>GIDPFTESVLQSQATELLQKKAQLVSFKIQGIMKRIFMGANTLEKFLSDENSAINDTLKRRMLSEFLLANPHVLLVSAIYTNNNERVITAMSMDSKIAYPNTT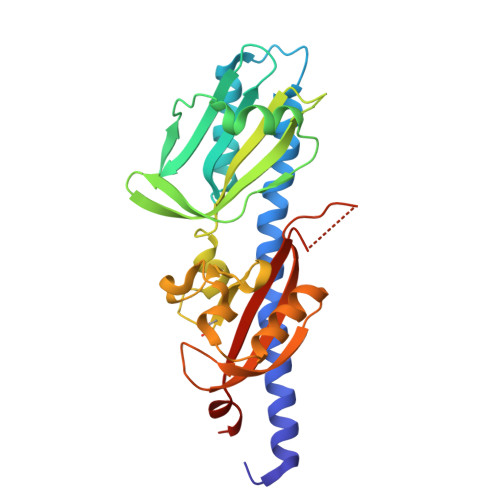LNENMTNQIRSLKSITHSDPYYKEVNGDKIYGMDITLPLMGKNQNAIGALNFFLNIDAFYTDVVGKKKSNTFLMGKDGRLLINPNREIQDKILSAINPDRRVAKAVEYYNQNEAGTLSYHSLSGNTETFLAIQPFDFFEEKGNNGNHWRWAIGKYVNKSLVFKEATN[3x]> GPSILEEYIRMAKNKEFFDALEEIAESAKNDETLRNELAKVLDDILKTDPSDPEAFRKIVAEHQEFWDEHDPSLMEFNEGRFFGKSRKQYLKSDDFLNSTDPTYNFQKLHQFAAEQRVKLGLEKSDTDTLVAILKNNPEECRAYIESKKPGLGNFSEGNVHGWLKEEYTPTIPPKAINKSTGVLSDEAI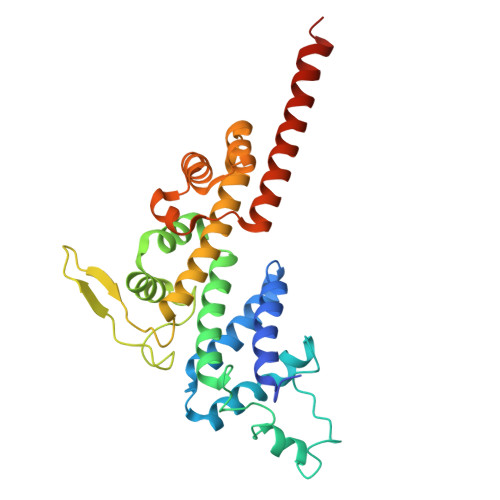KRIKEQARDLLLLKLINSSGNTQLLKDLRDAMSKPEAERAANALGFPTEGNGVLFLSREVVDALEERVEKLEQEAAKRGFDSYVQSLSHNALLA>[2x]GSHMTYPKYLLSPETIEALRKPTFDVWLW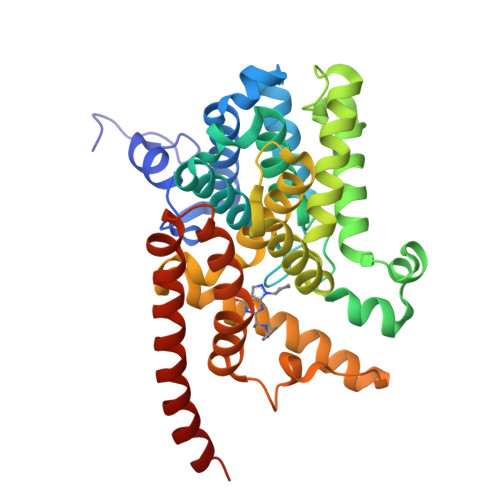EPNEMLSCLEHMYHDLGLVRDFSINPVTLRRWLFCVHDNYRNNPFHNFRHCFCVAQMMYSMVWLCSLQEKFSQTDILILMTAAICHDLDHPGYNNTYQINARTELAVRYNDISPLENHHCAVAFQILAEPECNIFSNIPPDGFKQIRQGMITLILATDMARHAEIMDSFKEKMENFDYSNEEHMTLLKMILIKCCDISNEVRPMEVAEPWVDCLLEEYFMQSDREKSEGLPVAPFMDRDKVTKATAQIGFIKFVLIPMFETVTKLFPMVEEIMLQPLWESRDRYEELKRIDDAMKELQKK>[2x]SN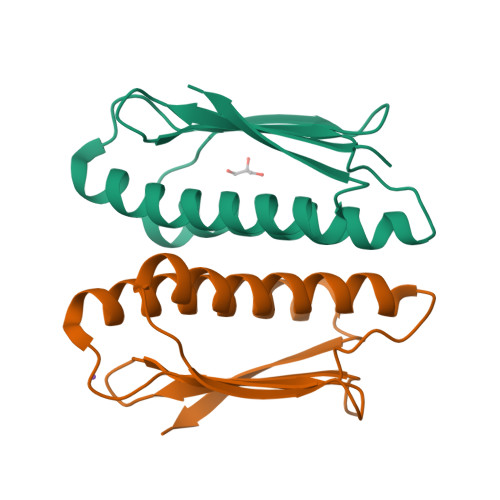AMIQAVFERAEDGELRSAEITGHAESGEYGLDVVCASVSTLAINFINSIEKFAGYEPILELNEDEGGYLMVEIPKDLPSHQREMTQLFFESFFLGMANLSENYSEFVQTRVITEN>[2x]MACPLEKALDVMVSTFHKYSGKEGDKFKLNKSELKELLTRELPSFLGKRTDEAA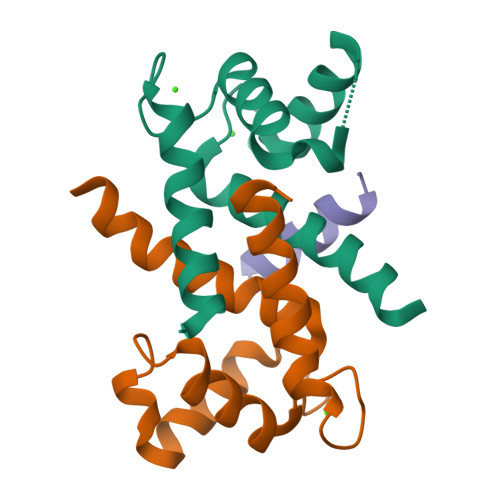FQKLMSNLDSNRDNEVDFQEYCVFLSCIAMMCNEFFEGF;> DAMNREVSSLKNKLRR3-chlorobenzothiophene-2-carbohydroxamic 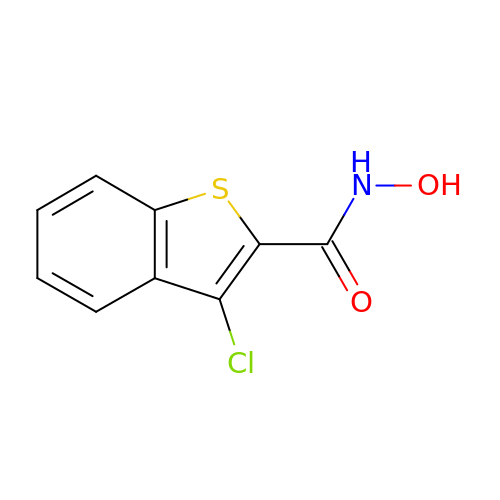acid | C9 H6 Cl N O2 S | HRXULFWGEYSULN-UHFFFAOYSA-N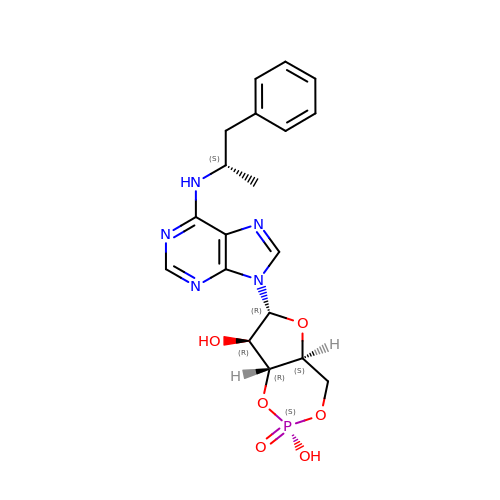(2S)-N6-(1-Methyl-2-phenylethyl)adenosine-3',5'-cyclic monophosphate | C19 H22 N5 O6 P | MKYZONTUKKUGCB-IQAYWSRLSA-N> MGDTGLRKRREDEKSIQSQEPKTTSLQKELGLISGISIIVGTIIGSGIFVSPKSVLSNTEAVGPCLIIWAACGVLATLGALCFAELGTMITKSGGEYPYLMEAYGPIPAYLFSWASLIVIKPTSFAIICLSFSEYVCAPFYVGCKPPQIVVKCLAAAAILFISTVNSLSVRLGSYVQNIFTAAKLVIVAIIIISGLVLLAQGNTKNFDNSFEGAQLSVGAISLAFYNGLWAYDGWNQLNYITEELRNPYRNLPLAIIIGIPLVTACYILMNVSYFTVMTATELLQSQAVAVTFGDRVLYPASWIVPLFVAFSTIGAANGTCFTAGRLIYVAGREGHMLKVLSYISVRRLTPAPAIIFYGIIATIYIIPGDINSLVNYFSFAAWLFYGLTILGLIVMRFTRKELERPIKVPVVIPVLMTLISVFLVLAPIISKPTWEYLYCVLFILSGLLFYFLFVHYK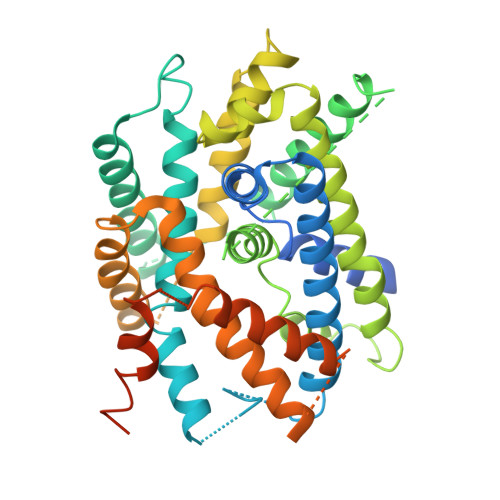FGWAQKISKPITMHLQMLMEVVPPEEDPE>[2x]GSDEAAELMQQVNVLKLTVEDLEKERDFYFGKLRNIELICQENEGENDPVLQRIV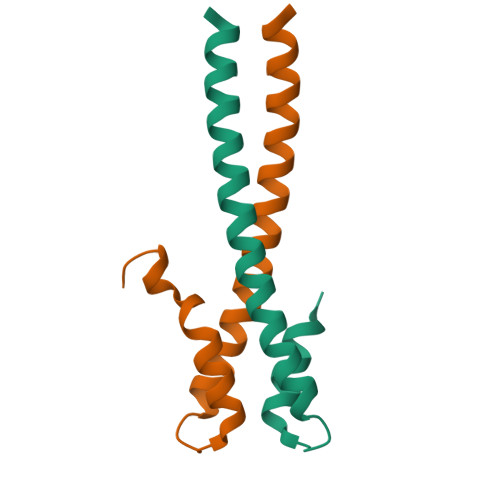DILYATDEGFVIPDEGGPQEEQEEY>[4x]MALGTSGVKIHPNGNSNQLGVQLENVKLTSLFKKLDKRCSLASWIKENIKKKECCFYVEDGREGICKCGYPKVQHCDEAIKPEDYMGEQWDKHRHVRETPTDAFGDISFGGLGQKTGKYVRVSSDTSCENLYQLMTEQWKLRSPNLLISVTGGAKNFYIKTHLKDKFRRGLIKVAQTTGAWILTGGTHAGVMKHVGMAVRDYTLSSGSMEGQIVVIGVAPWGVIHNRSTLIHPEGRFPAYYSLDEQGQGRLSCLDINHTHFLLVDDGTQGHYGVEIELRARLEKLISKLSLGNRESGVTIPVVCVVLDGGPGTLNTIYNSMLNHTPCVVLEGSGRLADVIAHVASVPVSKVTMALINRLLKRFFMQEYKNFTELQIIEWTKKIQDILRMPHLLTVFRIDEDKNYDVDVAILQALLKASRSDEHAGRHCWERQLELAVAWNRVDIAESEIFTEESQWTSSDLHPAMFSALVGDKPEFVRLLLENGVCVREFLEREETLCELYSHLPSCFFLRKLAKRVQGGKMRRGQEPLPGSRKVCLSHVSEEVRHLLGSFTQPLYIASRYKPTKDDVRLKVPSKGALDLPCSGEEWSADTVWDPGRDLFLWAVVQNNRELAEIGWEQCRDCIAAALAASKILRKLAQESGEDDSEEATEMLELANHYEKQAIGVFSECHSWDAQRAQKLLIRISPSWGRSTCLWLALEAHDKSFIAHSGVQALLTQIWCGELSVDNPHWKVLLCMIFFPLIYTGFLTFRRDEDIQRQAERTEQQKLAMESVFAGQSDGKIKRHLRGFSQKSELKPLNCSSRLMSFLKSPQVKFYWNIASYFGFLWLFAVVLMIDFQTSPSWRELLLYVWLTSLVCEEIRQLYHDFDGSGFRRKAKMYIKDLWNILDVLSIVLFIAGLICRLQASDTVFYIGKVILCIDFIIFCLRLMAIFSISRTLGPKIIIVRRMMLDLFFFMFLLSIWVVAYGVAKQGILIENEERLNWIIRGAVYEPYITIFGNFPTNIDNTLFDISSCSVNASDPLKPKCPMLNADNTPVFPEWLTIMMLCVYLLFANILLLNLLIAIFNYTFQEVQDNTDTIWKFQRYELIKEYHSRPALPPPFILLSHLILFIRGVFLRDLPQRHKNFRQELEQTEEEELLSWEAYMKDNYLASTRQDESQSVEHRIHDTAEKVGAMSELLEREQEMVXXXXXXXXXXXXXXXXXXXXXXDEEAPHMFARQLQYPDSTVRRFPVPEEKVSWEVNFSPYQPPVYNQQDSSESDTSALDKHRNPGGRTGIRGKGALNTLGPNHILHPIFTRWRDAEHKVLEFLAVWEDAEKRWALLGGPAQPDEPLAQVLERILGKKLNEKTKTLLKAGEEVYKGYVDDSRNTDNAWVETSIITLHCDKNTPLMADLNHMVESSLSSHQPLQWREVSSDACRCSYQREALRQIAHHHNTYFSNSLEVLFQGPDYKDDDDKAHHHHHHHHHH

TRPM2 is a calcium-permeable nonselective cation channel that is widely expressed in the nervous, immune, and endocrine systems, and plays a crucial role in warmth and redox-dependent signaling. Extensive electrophysiological studies have shown that activation of TRPM2 by ROS is caused by an increase of intracellular ADP-ribose (ADPR), a TRPM2 agonist, and that both ADPR and Ca2+ are required for channel activation. Our TRPM2DR channel forms a homo-tetramer. Similar to the previously reported TRPM2, TRPM4, and TRPM8 structures, each TRPM2DR protomer contains an N-terminal region composed of MHR1 to MHR4, a transmembrane channel region, and a C-terminal region.

In contrast to the canonical four-fold symmetry reported in the TRPM2closed and TRPM2open structures and the pseudo four-fold symmetry observed in the TRPM2DR_Apo structure, our TRPM2DR_Ca2+ structure adopts pronounced two-fold symmetric arrangements when viewed along the central axis of the channel. The symmetry reduction from C4 to C2 is most pronounced in the middle layer of the CD, which comprises the MHR1/2 and MHR3 domains, giving rise to conformationally distinct protomers within our TRPM2DR_Ca2+ structure. Notably, protomers A and C adopt a conformation that is consistent with the published TRPM2closed structure, while B and D resemble TRPM2open. While the MHR3, MHR4, and VSLD are conformationally similar across protomers, substantial domain arrangements are observed at three junctions: NUDT9H-MHR1/2, MHR1/2-MHR3, and VSLD-pore. In protomer A, the S4b adopts a 310-helical structure, while the equivalent region in protomer B contains an α-helical structure and an unstructured loop. In addition, the S4–S5 linker in protomer A contains a π-helix, while the corresponding region in protomer B is α-helical and forms a continuous straight helix with S5. Although the distances between diagonally opposed gate residues in TRPM2DR_Ca2+ are larger than those observed in the TRPM2closed structure, the S6 gate in TRPM2DR_Ca2+ is not as wide as that observed in the TRPM2open structure. Whereas the NUDT9H and MHR1/2 domains in protomer A exhibit only intra-subunit interactions, the core subdomain of the NUDT9H in protomer B makes additional contacts with the MHR1/2 domain in the neighboring protomer, resembling the interaction networks depicted in the TRPM2closed and TRPM2open structures, respectively. Consistent with this idea, the density for Ca2+ in the TRPM2DR_Ca2+ reconstruction is stronger in protomer B than in protomer A (10.8 σ versus 9.5 σ, respectively). Second, endogenous ADPR happened to be captured in the Ca2+-bound TRPM2 during sample preparation, as we also observe weak densities in the cleft of the MHR1/2 domain in protomers B and D of the TRPM2DR_Ca2+ reconstruction, which may correspond to ADPR.> SMGEVVMSQAIQPAHATARGELSAGQLLKWIDTTACLAAEKHAGVSCVTASVDDIQFEETARVGQVITIKAKVTRAFSTSMEISIKVMVQDMLTGIEKLVSVAFSTFVAKPVGKEKIHLKPVTLLTEQDHVEHNLAAERRKVRLQHEDTFNNLMKESSKFDDLIFDEEEGAVSTRGTSVQSIELVLPPHANHHGNTFGGQIMAWMETVATISASRLCWAHPFLKSVDMFKFRGPSTVGDRLVFTAIVNNTFQTCVEVGVRVEAFDCQEWA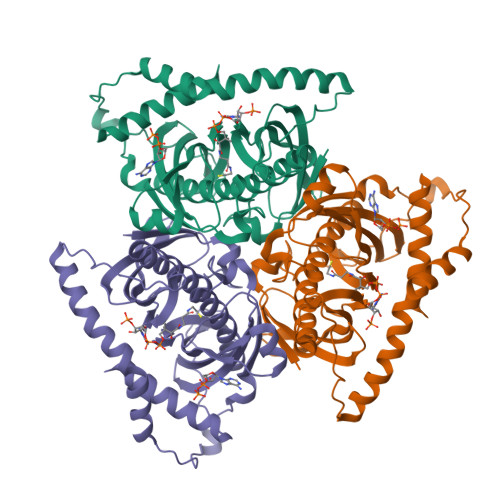EGRGRHINSAFLIYNAADDKENLITFPRIQPISKDDFRRYRGAIARKRIRLGRKYVISHKEE> SVYTYFSAVAGQDGEVDAEEL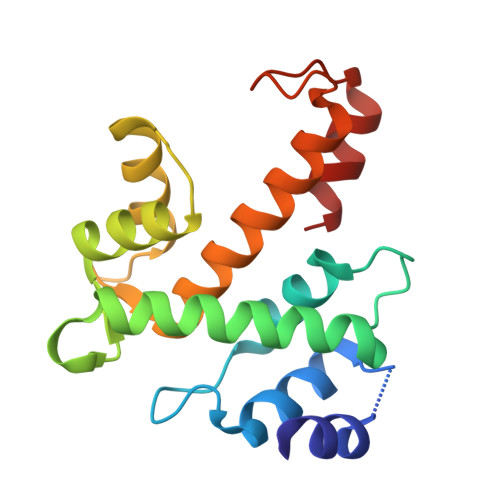QRCLTQSGINGTYSPFSLETCRIMIAMLDRDHTGKMGFNAFKELWAALNAWKENFMTVDQDGSGTVEHHELRQAIGLMGYRLSPQTLTTIVKRYSKNGRIFFDDYVACCVKLRALTDFFRKRDHLQQGSANFIYDDFLQGTMAI>MSERHLFTSESVSEGHPDKIADQISDAILDAMLAQDPQARVAVETSVTTGLVLVFGEVSTKAYVDIQKVVRDTIKSIGYVDGQYGFDGDNCAVLVSLDEQSPDIAQGVDDSLETRSGDADPLDQIGAGDQGMMFGYAINETPELMPLPIALSHRLMRKIAALRKDGTIKWLRPDAKAQVTVEYDEDNQPKRIDTVVLSTQHDPDVDLDTIRQTVIDQVIKAVLPADLLDDQTKYLVNPTGRFVIGGPQGDAGLTGRKVIVDTYGGFAHHGGGAFSGKDATKVDRSASYAARYIAKNVVAAGLADQVEVQLAYAIGVAEPVSIAVDTAGTGKVSDEALINAIRENFDLRPAGIIKMLDLQRPIYRQTAAYGHFGRTDIDLPWEHTDKVDALKAAFKHHHHHH[8x]

MATs are an essential and ubiquitous enzyme family found in all domains of life. 38 MATs catalyze the condensation of ATP with methionine to generate S‐adenosylmethionine (SAM)—an essential molecule involved in numerous biological processes, including RNA, DNA, protein and small molecule methylation, polyamine synthesis, and production of enzyme cofactors. 39 Analysis of available crystal structures reveals that bacterial MATs are predominantly dihedral homotetramers (D2 symmetry group), that is, comprised of dimers of dimers 40. Two deep cavities harboring active sites are located directly in this dimeric interface, making the homodimer the obligatory functional unit.

To enrich the structural dataset, we determined the crystal structure of MAT from Lactiplantibacillus planatrum at 2.82 Å resolution, making it the only current MAT representative of the Bacillota phylum, and added this structure to analysis. We also found that MAT from Lactiplantibacillus plantarum (LpMAT) does not require chaperonins for folding and activity. Similarly to NgMAT, LpMAT assumes a predominantly dimeric state in solution, its interdimeric interface lacks salt‐bridges, and is less hydrophobic than EcMAT. Since MATs from N. gonorrhoeae and L. plantarum fold and assemble in the absence of chaperonins, the folding dependency of EcMAT is not a general inherent property of the MAT fold.>[2x]GPLGSPEFGYWITCCPTCDVDINTWVPFYSTELNKPAMIYCSHGDGHWV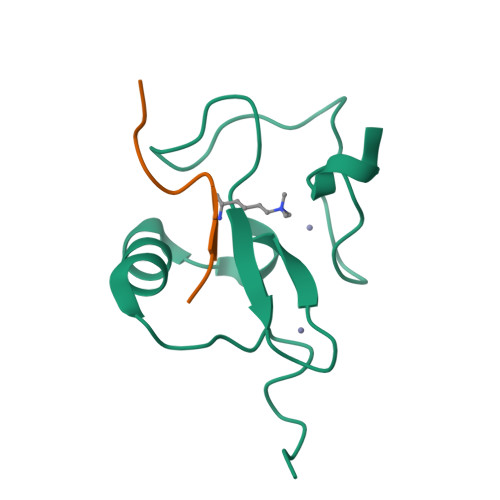HAQCMDLEERTLIHLSEGSNKYYCNEHVQIARA;>[2x]ARTKQTAAKA> GSHMGSPNSPLKDSLRPKLSEEQQHIIAILLDAHHKTYDPTYADFRDFRPPVRMDGSTGSVTLDLSPLSMLPHLADLVSYSIQKVIGFAKMIPGFRDLTSDDQIVLLKSSAIEVIMLRSNQSFTMDDMSWDCGSQDYKYDVTDVSKAGHTLELIEPLIKFQVGLKKLNLHEEEHVLLMAICIVSPDRPGV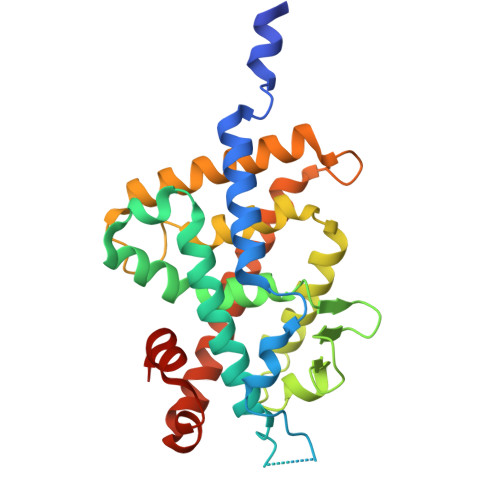QDAKLVEAIQDRLSNTLQTYIRCRHPPPGSHQLYAKMIQKLADLRSLNEEHSKQYRSLSFQPENSMKLTPLVLEVFGNEIS>MSFSMVTRYAHSPEDIQHYDTSKLRHEFLMEKIFNPGDILLTYTYNDRMIFGGVMPTDEPLEIKLSTELGVDFFLQRRELGIINIGGAGAITIDGRKDAMSNQDGYYIGMGTQKVVFTSEDRDHPAKFYVVSTPAHKTYPNKKLPFATALAKPMGDQQHLNKRTIYKYIDASQMDT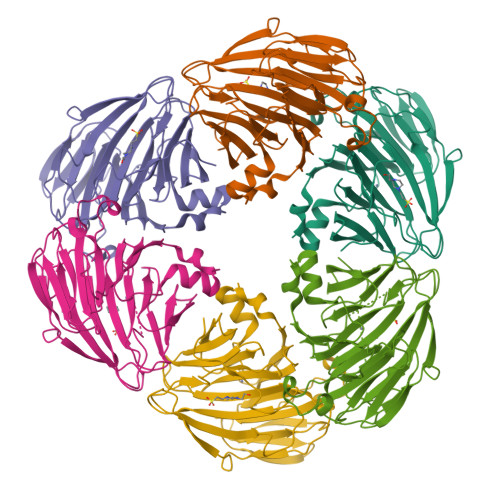CQLQMGYTVLEPGSSWNTMPAHTHARRMETYMYFNFADPETRVFHFLGKPDETRHITLFNEQAVVNPSWSIHCGVGTTNYAFIWAMCGENQTYDDMDQVAMNELRLEHHHHHH[6x]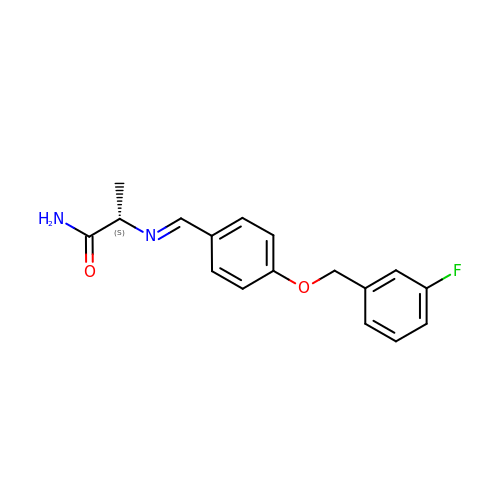(S)-(+)-2-[4-(FLUOROBENZYLOXY-BENZYLAMINO)PROPIONAMIDE] | C17 H17 F N2 O2 | RJJDIVMWGWHPFE-QDBSGRMGSA-N Transthyretin (TTR)3 is a 55-kDa protein that aggregates into amyloid fibrils under pathological conditions. In its native tetrameric conformation, TTR transports retinol-binding protein and thyroxine (T4) in the blood and cerebrospinal fluid. Amyloid aggregation of TTR occurs by dissociation of tetrameric TTR into monomers; these partially unfold into amyloidogenic intermediates and self-associate into soluble oligomers and amyloid aggregates. Here we identify two segments of TTR that drive protein aggregation by self-association and formation of steric zipper spines of amyloid fibrils.

To better understand how 91AEVVFT96 self-associates to form fibrils, we determined the structure of the fibril-like crystals of 91AEVVFT96. We found that it forms a Class-7 steric zipper (Ref. 25 and Fig. 2D) in which the β-strands stack into antiparallel β-sheets with identical side chains on both faces. In addition, to further prove that β-strands F and H can participate in amyloid core formation of TTR fibrils, we determined the crystal structure of the steric zippers formed by the segments in isolation by x-ray crystallography. The crystal structure of 91AEVVFT96 revealed a Class-7 steric zipper with antiparallel β-strands and antiparallel sheets (Ref. 25 and Fig. 2D). The side chain organization explains why the residue replacements E92P and V94P hinder TTR aggregation because the proline substitution would decrease the shape complementarity between sheets in the steric zipper structure. In the isolated segment 91AEVVFT96, proline replacements in positions 92 and 94 completely prevented fibrillization.

>[2x]AEVVFT>MGSMISTPEPLHAGHILTPFCCGVDSIDNWLKQRAMKNQTTGASRTFVCCGSDSNVLAYYSLASSAVTTNTSPGRFRRNMPDPIPVVVLGRLAVDKSLHGQGVARALVRDAGLRVIQVAETIGIRGMLVHALSDEAREFFQRVGFVPSPMDPMMLMVTLGDLVESV[2x];>GSMPAANSMAMKRETLNLRIKPAERDLIDRAAKARGKNRTDFVLEAARAAAEEALIEQR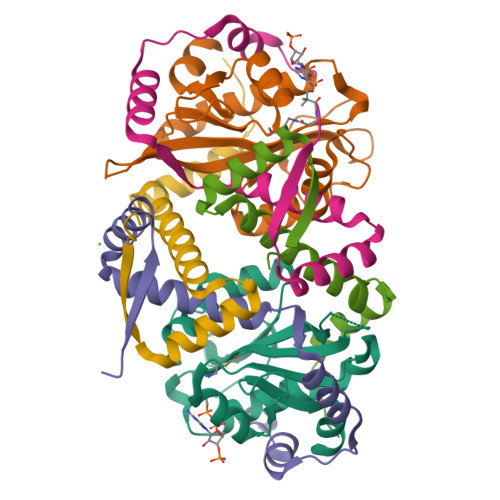IIMADPEAYQEFLVRLDQTPSPNAALRKTMQTPAPWEQEK[4x]1-[2-[(1~{R},3~{S},5~{R})-3-[[(1~{R})-1-(3-chloranyl-2-fluoranyl-phenyl)ethyl]carbamoyl]-2-azabicyclo[3.1.0]hexan-2-yl]-2-oxidanylidene-ethyl]pyrazolo[3,4-c]pyridine-3-carboxamide 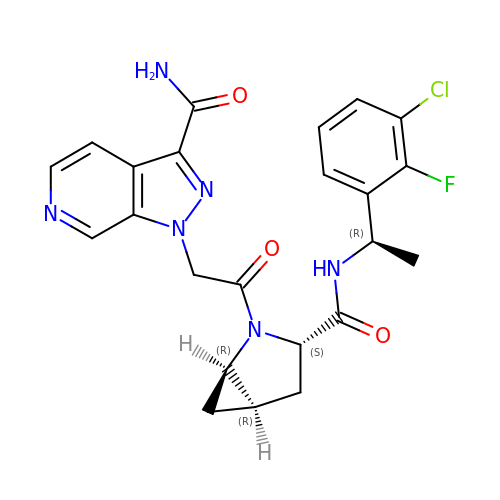| C23 H22 Cl F N6 O3 | YAALCKJNOOFODD-SKNMWMDOSA-N>[6x]MSLAFTKTRSTIGIVAQPVSVEVHLSNGLPSFTMVGLAETAVKESKDRVRSAIINSQFEFPCRKITVNLGPANLPKTGSGFDLPIALGILAASEQIPLTNLANHEFIGELALSGELRGVSAIIPAVLAAHKDNQHLIIANANAAEASLTGHQKVFTANNLREVCDYLCQGTSLQSLPPKPDLLLNNYELDWSDIKGQQHAKNAMVIAACGGHSILLSGAPGSGKTMMAKRFSTLLPELSETQALECAAINSIRGKLPDFREWRLPPFRAPHHTASPVALVGGGNPPKPGEISLAHHGVLFLDELPEFNRQVLETLREPLESGHICISRAAAQIEFPAKFQLIAAMNPCPCGQWGNS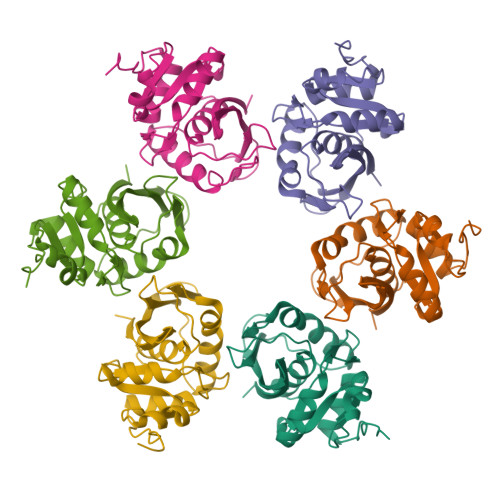QANCMCTPDRISRYLAKLSAPLLDRIDMQVTIHALSQEELIKPNTHLEKQSLAIREKVTKMHEIQMARQDSLNANLNSKTCEMVCELGSEEQLFLREVMSKLKLSARGYHRLLKVSRTIADMNSSKKVLLNHLQQALSYKQNLHLPKHHHHHH> GDTKEQRILNHVLQHAEPGNAQSVLEAIDTYCEQKEWAMNVGDKKGKIVDAVIQEHQPSVLLELGAYCGYSAVRMARLLSPGARLITIEINPDCAAITQRMVDFAGVKDKVTLVVGASQDIIPQLKKKYDVDTLDMVFLDHWKDRYLPDTLLLEECGLLRKGTVLLADNV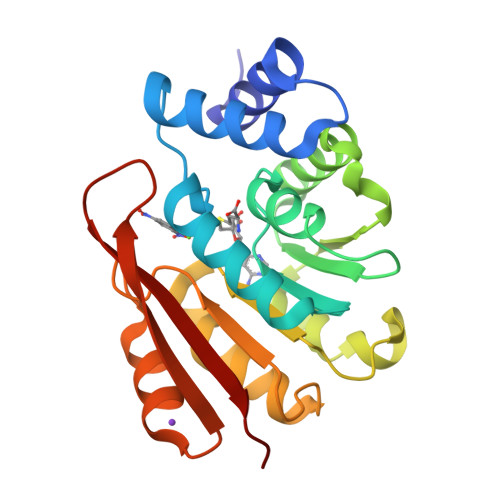ICPGAPDFLAHVRGSSCFECTHYQSFLEYREVVDGLEKAIYKGP4-Chlorophenacyl-coenzyme A | 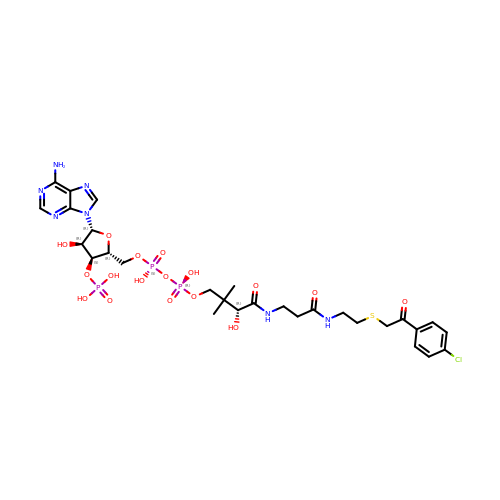C29 H41 Cl N7 O17 P3 S | JKZHFXZXNBMAGG-VXAHOBLNSA-N>GGFQVVTFEWAHVQDPYVIALWILVASLAKIGFHLSHKVTSVVPESALLIVLGLVLGGIVWAADHIASFTLTPTVFFFYLLPPIVLDAGYFMPNRLFFGNLGTILLYAVVGTVWNAATTGLSLYGVFLSGLMGDLQIGLLDFLLFGSLMAAVDPVAVLAVFEEVHVNEVLFIIVFGESLLNDAVTVVLYNVFESFVALGGDNVTGVDCVKGIVSFFVVSLGGTLVGVVFAFLLSLVTRFTKHVRIIEPGFVFIISYLSYLTSEMLSLSAILAITFCGICCQKYVKANISEQSATTVRYTMKMLASSAETIIFMFLGISAVNPFIWTWNTAFVLLTLVFISVYRAIGVVLQTWLLNRYRMVQLEPIDQVVLSYGGLRGAVAFALVVLLDGDKVKEKNLFVSTTIIVVFFTVIFQGLTIKPLVQWLKVKRSEHREPRL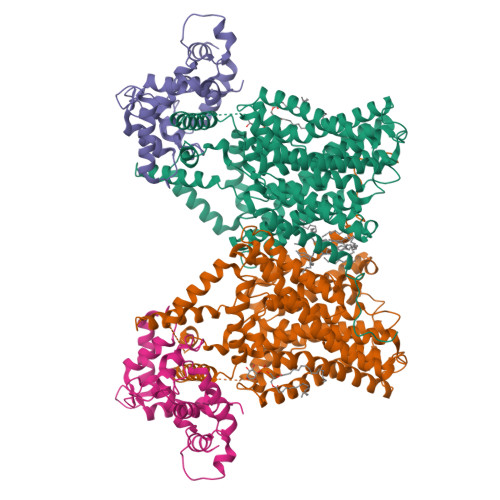NEKLHGRAFDHILSAIEDISGQIGHNYLRDKWSHFDRKFLSRVLMRRSAQKSRDRILNVFHELNLKDAISYVAEGERRGSLAFIRSPSTDNVVNVDFTPRSSTVEASVSYLLRENVSAVCLDMQSLEQRRRSIRDAEDMVTHHTLQQYLYKPRQEYKHLYSRHELTPTEDEKQDREIFHRTMRKRLESFK[2x];>[2x]DEELEEIKKETGFSHSQITRLYSRFTSLDKGENGTLSREDFQRIPELAINPLGDRIINAFFPEGEDQVNFRGFMRTLAHFRPIEDNEKSKDVNGPEPLNSRSNKLHFAFRLYDLDKDEKISRDELLQVLRMMVGVNISDEQLGSIADRTIQEADQDGDSIASFTEFVKVLEKVDVEQKMSIRFLH>[4x]MYGKLLICAT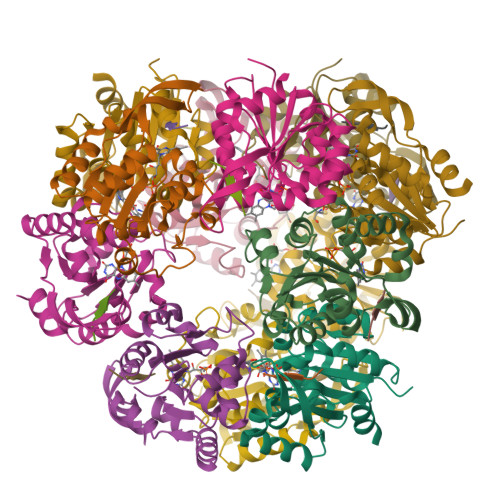ASINVININHYIVELKQHFDEVNILFSPSSKNFINTDVLKLFCDNLYDEIKDPLLNNINIVENHEYILVLPASANTINKIANGICDNLLTTVCLTGYQKLFIFPNMNIRMWGNPFLQKNIDLLKNNDVKVYSPDMNKSFEISSGRYKNNITMPNIENVLNFVLNNEKRPLD;>DSYTC[4x]> MRGSHHHHHHGSMAAAAELSLLEK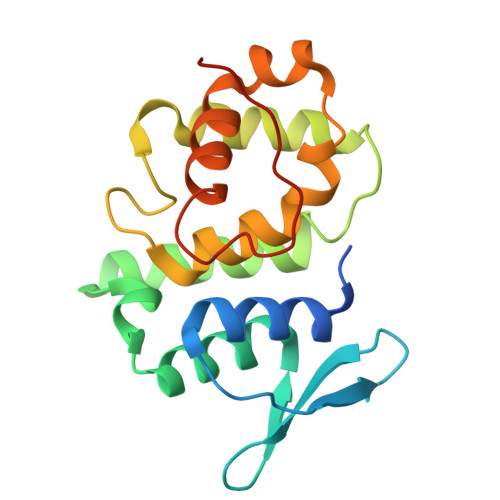SLGLSKGNKYSAQGERQIPVLQTNDGPSLTGLTTIAAHLVKQANKEYLLGSTAEEKAIVQQWLEYRVTQVDGHSSKNDIHTLLKDLNSYLEDKVYLTGYNFTLADILLYYGLHRFIVDLTVQEKEKYLNVSRWFSHIQHYPGIRQHLSSVVFIKNRLYTNSH>SNATNTDTNSTNNSPNNTTNTTTNVTTTSDKNTIPIGIALAQTSNVALLGQEQVAGAKIAEKYFNDKGGVNGTPIKLIFQDTAGDEAGTINAFQTLINKDKVVGIVGPTLSQQAFSANPIAERAKVPVVGPSNTAKGIPEIGDYVARVSAPVSVVAPNSVKAALKQNPNIKKVAVFFAQNDAFSKSETEIFQQTVKDQGLELVTVQKFQTTDTDFQSQATNAINLKPDLVIISGLAADGGNLVRQLRELGYQGAIIGGNGLNTSNVFAVCKALCDGVLIAQAYSPEYTGEINKAFRQAYVDQYKKEPPQFSAQAFAAV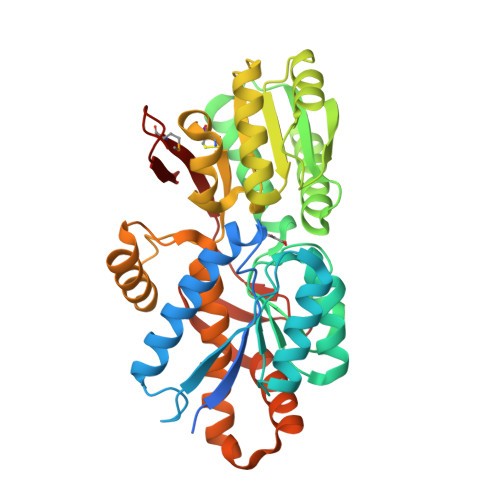QVYVESLKALDTKNKVSKIQLPELRTELNKQLLTGKYNTPLGEISFTPIGEVVQKDFYVAQIKMEKDGSQGKFTFLK[2x]>[5x]MSLLSDLCNLNLSESTEKIIAEYIWIGGSGMDLRSKARTLNAPVSDPSKLPQWNYDGSSTGQAPGEDSEVILYPQAIYKDPFRRGNNILVMCDAYTPGGEPIPTNKRFDAAKIFSHPDVVAEEPWYGIEQEYTLLQKEVKWPIGWPVGGYPGPQGPYYCGIGADKAFGRDIVDAHYKACLYAGINISGINGEVMPGQWEFQVGPSVGISSGDQLWMARYILERITEIAGVVVSFDPKPIEGDWNGAGAHTNYSTKSMRSDGGFEVIKKAIEKLGLKHREHIAAYGEGNERRLTGKHETADINTFLWGVANRGASIRVGRDTEKAGKGYFEDRRPASNMDPYIVTSMIANTTILWKP

One such an example is glutamine synthetases (GSs) (EC 6.3.1.2), one of the most ancient functioning enzymes in existence and a central enzyme in nitrogen metabolism of all living organisms, catalyzing the formation of glutamine by condensation of glutamate with ammonia using ATP as an energy source. Decades of studies have established a striking notion that all three classes of GS enzymes, despite of dramatic differences in amino acid sequences and protein sizes, share quaternary geometry in dihedral symmetry assembled with two oligomeric rings. Considering that the active sites of GS are located at the clefts formed between two neighboring protomers within the same ring and distal to the ring-ring interface, each isolated GS subcomplex ring holds multiple integral catalytic sites. Cryo-EM structure determination of GS in both the catalytically active and inactive assembly states allows us to reveal an unanticipated self-assembly-induced disorder-order transition paradigm, in which the remote interactions between two subcomplex entities significantly rigidify the otherwise structurally fluctuating active sites, thereby regulating activity.

In order to elucidate the mechanism of how the pentameric CsGSIb (thereafter named as CsGSIbPen) demonstrates distinct enzymatic properties than CsGSIbDec, we next determined the structure of CsGSIbPen. Lowering the sample concentration, which favored pentamer dissociation, allowed us to obtain sufficient number of CsGSIbPen particles (Figure 3—figure supplements 2 and 3), which, in turn, enabled us to solve the cryo-EM structure of the inactive single-ringed GSII for the first time. Unexpected, CsGSIbPen exhibited high conformational heterogeneity and 3D particles classification generated three similar structures with the r.m.s.d. ranging from 0.6 to 0.8 Å, differing in a few peripheral regions. The most striking difference between CsGSIbPen and CsGSIbDec is that several regions are missing in the electron density map of all three classifications of CsGSIbPen particles, with only 229–255 out of 356 residues electron densities in presence. As a result, CsGSIbPen demonstrated a decagram-shaped density map with a few regions missing at the rim, in sharp contrast to a pentagon-shaped map yielded by the CsGSIbDec particles. For the 229–255 residues that show clear density in CsGSIbPen particles, the conformation of each subunit in three CsGSIbPen EM structures, as well as the arrangement pattern, closely resembles that of the CsGSIbDec, as evidenced by r.m.s.d. in the range of 0.7–1.0 Å. The density-missing regions include the segments around residues of 110–117, 140–166, and 260–334, among which, the fragment around residues 260–334 is a major component making up an integral catalytic site, while the segment of residues 140–166 comprising of the two gear teeth is responsible for ring-ring interaction (–4d).2-AMINOBENZOIC ACID | C7 H7 N O2 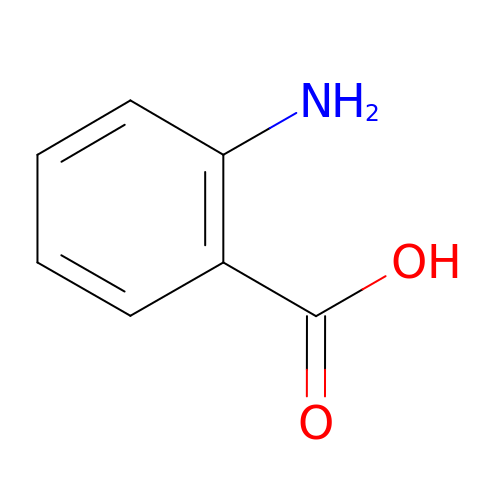| RWZYAGGXGHYGMB-UHFFFAOYSA-N YgjG is a putrescine aminotransferase (PATase, EC 2.6.1.82). Based on its amino acid sequence alignment, it belongs to the class III pyrodoxal-5′-phosphate (PLP)-dependent aminotransferase family, which include ornithine aminotransferase (OAT) and GABA aminotransferase (GABA-AT). In this study, we determined the crystal structures of YgjG from E. coli in free and putrescine-bound states at 2.3 and 2.1 Å resolutions, respectively, to investigate the structural basis of YgjG substrate specificity. The monomer comprises an N-terminal domain, a large PLP-binding domain, and a C-terminal domain.

The structure of YgjG in complex with PLP and putrescine was determined at 2.1 Å resolution. The putrescine electron density was observed in three of the four subunits in the asymmetric unit. The putrescine amino group bound the PLP at two of the three active sites. The covalent bond between PLP and Lys300 was broken, and the Lys300 side chain was displaced distal to the cofactor. The weak putrescine electron density could be explained by partial occupancy in the binding site and/or substrate flexibility. Putrescine binding to YgjG is mediated by a number of polar and hydrophobic interactions. The substrate N1 nitrogen atom forms hydrogen bonds with the Glu243 OE1 oxygen atom and the PLP O3 oxygen atom. The substrate N2 nitrogen atom was stabilized by a hydrogen bond with Gln119*. The putrescine was also surrounded by several residues, including Phe91, Phe180, Leu419 and Thr332*, which contributed to hydrophobic interactions with the substrate. The overall structure of YgjG in complex with putrescine was almost identical to the unbound YgjG (r.m.s. deviations value 0.34 Å over 452 Cα atoms), which indicates no significant movement at the domain level upon substrate binding, in contrast to aspartate aminotransferase.

>[4x]MNRLPSSASALACSAHALNLIEKRTLDHEEMKALNREVIEYFKEHVNPGFLEYRKSVTAGGDYGAVEWQAGSLNTLVDTQGQEFIDCLGGFGIFNVGHRNPVVVSAVQNQLAKQPLHSQELLDPLRAMLAKTLAALTPGKLKYSFFCNSGTESVEAALKLAKAYQSPRGKFTFIATSGAFHGKSLGALSATAKSTFRKPFMPLLPGFRHVPFGNIEAMRTALNECKKTGDDVAAVILEPIQGEGGVILPPPGYLTAVRKLCDEFGALMILDEVQTGMGRTGKMFACEHENVQPDILCLAKALGGGVMPIGATIATEEVFSVLFDNPFLHTTTFGGNPLACAAALATINVLLEQNLPAQAEQKGDMLLDGFRQLAREYPDLVQEARGKGMLMAIEFVDNEIGYNFASEMFRQRVLVAGTLNNAKTIRIEPPLTLTIEQCELVIKAARKALAAMRVSVEEALEHHHHHH One example is cyclohexadienyl dehydratase (CDT), which is closely related to the polar and cationic amino acid-binding proteins, such as the arginine-binding protein (ArgBP). Like ArgBP, CDT adopts a periplasmic type-II SBP fold, but instead of binding amino acids, it catalyzes the Grob-like fragmentation of prephenate and L-arogenate to form phenylpyruvate and L-phenylalanine, respectively. We previously used ancestral sequence reconstruction to show that the trimeric CDT from Pseudomonas aeruginosa (PaCDT) plausibly evolved from a monomeric cationic amino acid-binding protein ancestor (AncCDT-1) via a series of intermediates (AncCDT-2 to AncCDT-5)40. In this work, we have studied the structural dynamics of a series of states along an evolutionary trajectory from an ancestral L-arginine solute-binding protein (AncCDT-1) to an extant dehydratase (PaCDT).

In this work, we have additionally assessed the dehydratase activity of AncCDT-5, which proved to be an intermediate between the AncCDT-3 variants and the extant enzyme PaCDT. Although the kcat value of AncCDT-5 (4 s−1) exceeds the level observed in the AncCDT-3 variants (~10−2 s−1) almost as much as PaCDT (18 s−1), the KM of AncCDT-5 remains ~15-fold higher than that of PaCDT (277 μM vs. 19 μM). To better understand how the mutations along this evolutionary trajectory affect activity, we also solved a 1.49 Å X-ray crystal structure of AncCDT-5, which shares 15/15 residues in the active/substrate-binding site with PaCDT. Since these active/binding sites are identical, the ~15-fold decrease in KM and ~5-fold increase in kcat of the dehydratase activity must be attributed to amino acid substitutions that are outside of the binding site. Unlike the wide-open crystal structure of AncCDT-3/L188, the 1.49 Å crystal structure of AncCDT-5 determined in this work adopts the closed conformation (a HEPES molecule is bound in the active site), with a Q68-R138 Cα–Cα distance of 2.8 nm (Gd(III)–Gd(III) distance: 3.1 nm). Beginning from this closed state, we again performed triplicate 500 ns MD simulations after removing the HEPES molecule. The simulations predict that the protein rapidly adopts a wide-open conformation, with a Q68-R138 Cα–Cα distance range of 3.6–4.2 nm (Gd(III)–Gd(III) distance range: 4.5–5.4 nm) that is analogous to the wide-open conformation seen in the MD simulations of AncCDT-1, the crystal structure of the L-arginine-binding protein from T. maritima, and the crystal structure of AncCDT-3. Likewise, AncCDT-5 displayed the most prominent distance-distribution peak at ~5.4 nm. The combination of the DEER, crystallographic and MD data for the experiments performed on AncCDT-3 and AncCDT-5 suggest that both proteins predominantly access a wide-open state in solution.

> GIAASRLDEIMQRGTLRVGTTGDYKPFSYRDPDGQFTGFDIDMAESLAKSLGVKVEFVPTTWPTLMDDFQADKFDIAMGGVSVTPERQKKADFSEPYMTDGKTPIVRCEDADKYQTLEQIDRPDVRVVVNPGGTNERFARAHLKQAQITVYPDNVTIFQEIVAGRADVMMTDAVETRYQQKLHPGLCAVHVDKPFTHSEKAYLLPRGDPAFKAYVDQWLHQAMQSGTYQRIFDKWLKL> MSFKATITESGKQNIWFRAIYVLSTIQDDIKITVTTNELIAWSMNETDTTLCQVRFQKSFFEEYEFKPHEIVFGENGVQVIEDTYGNSHKLYSFRVNGRHLTTISRKPDGDGIKSFTIAVNNTSTCPESLANRLIVVIEMDSLIVKEYCPQFQPIKYDPIIINLKYKRRFLDVFGTAASDRNPQEPLDPKLLDVFTNTERELTSALFNEEVESDIRKRNQLTAADEINYICCNSTLLKNFLDNCNVNVTDEVKLEINVHRLSITAFTKAVYGKNNDLLRNALSMSNTISTLDLEHYCLFTTIEDEKQDKRSHSKRREHMKSIIFKLKDFKNFITIGPSWKTTQDGNDNISLWFCHPGDPILMQMQKPGVKLELVEVTDSNINDDILEGKFIKTAISGSKEEAGLKDNKESCESPLKSKTALKRENLPHSVAGTRNSPLKVSYLTPDNGSTVAKTYRNNTARKLFVEEQSQSTNYEQDKRFRQASSVHMNMNREQSFDIGTTHEVACPRNESNSLKRSIADICNET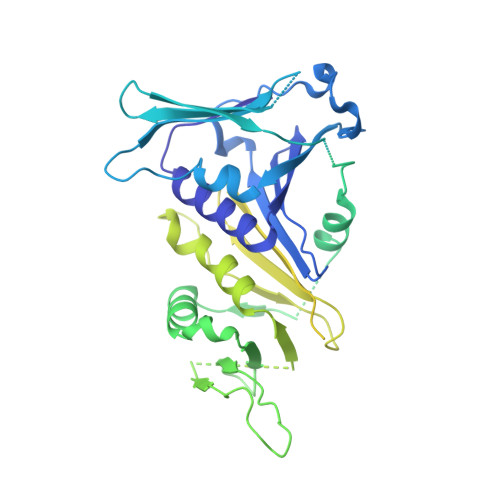EDPTQQSTFAKRADTTVTWGKALPAADDEVSCSNIDRKGMLKKEKLKHMQGLLNSQNDTSNHKKQDNKEMEDGLGLTQVEKPRGIFD Parasite-infected red blood cells sequester in the placenta through interaction between parasite-expressed protein VAR2CSA and the glycosaminoglycan chondroitin sulfate A (CS) abundantly present in the intervillous space. Here, we report cryo-EM structures of the VAR2CSA ectodomain at up to 3.1 Å resolution revealing an overall V-shaped architecture and a complex domain organization. Compared to other PfEMP1s, the ~310 kDa VAR2CSA ectodomain is relatively conserved among parasites. It is composed of a short N-terminal segment and six Duffy Binding-Like (DBL) domains (DBL1-DBL6) unique to VAR2CSA. Several of the DBL domains are linked by complex inter-domain (ID1-3) regions with limited or no homology among PfEMP1s yielding a DBL1-ID1-DBL2-ID2-DBL3-DBL4-ID3-DBL5-ID4-DBL6 structure.

The extracellular region from the N-terminal methionine (M1) to amino acid F2649 representing the entire ectodomain of the FCR3 VAR2CSA variant was expressed in baculovirus transfected insect cells as a secreted monomeric protein and purified by immobilized nickel affinity chromatography. As the binding to CSPG in NaCl buffer showed a 1:2 stoichiometry compared to a 1:1 in KCl buffer, the less compact VAR2CSA could introduce more unspecific binding or the proposed additional minor groove binding site is more exposed in NaCl buffer allowing CSPG binding. Structural analysis was performed in KCl buffer, as the highest affinity toward CSPG was observed. Next, we determined the cryo-EM structure of the isolated VAR2CSA form generated from a map of overall 3.8 Å resolution. The final model represents the ectodomain of VAR2CSA, exhibiting a well-folded conformation with clearly defined DBL domains and in agreement with previously published structures of DBL3, DBL4 and DBL6. The region spanning ID1-DBL2-ID2-DBL3-DBL4-ID3 represents the core of the macromolecular structure, as highlighted by a compact structure with a high degree of inter-domain interactions. The structure discloses the fold of ID2, forming a separate domain consisting of a bundle of α-helices, a shape which together with ID3, a 30 residues long α-helix (residue 1955-1985), serves as a structural glue for the core. Notably, ID2 and ID3 interact, as the C-terminus of ID2 forms an open-mouth shape conformation, which interacts extensively with the ID3 α-helix. DBL1 exhibits only a few inter-domain interaction sites with DBL2 and DBL4, leaving a cleft in-between the core and DBL1. The similarity of the VAR2CSA FCR3 apo-structures by Ma et al., and the one presented here is high, with RMSD in the core region (AA residue 450–2022) of 1.38 Å.

> MDSTSTIANKIEEYLGAKSDDSKIDELLKADPSEVEYYRSGGDGDYLKNNICKITVNHSDSGKYDPCEKKLPPYDDNDQWKCQQNSSDGSGKPENICVPPRRERLCTYNLENLKFDKIRDNNAFLADVLLTARNEGEKIVQNHPDTNSSNVCNALERSFADLADIIRGTDQWKGTNSNLEKNLKQMFAKIRENDKVLQDKYPKDQKYTKLREAWWNANRQKVWEVITCGARSNDLLIKRGWRTSGKSDRKKNFELCRKCGHYEKEVPTKLDYVPQFLRWLTEWIEDFYREKQNLIDDMERHREECTREDHKSKEGTSYCSTCKDKCKKYCECVKKWKTEWENQENKYKDLYEQNKNKTSQKNTSRYDDYVKDFFEKLEANYSSLENYIKGDPYFAEYATKLSFILNPSDANNPSGETANHNDEACNCNESGISSVGQAQTSGPSSNKTCITHSSIKTNKKKECKDVKLGVRENDKDLKICVIEDTSLSGVDNCCCQDLLGILQENCSDNKRGSSSNDSCDNKNQDECQKKLEKVFASLTNGYKCDKCKSGTSRSKKKWIWKKSSGNEEGLQEEYANTIGLPPRTQSLYLGNLPKLENVCEDVKDINFDTKEKFLAGCLIVSFHEGKNLKKRYPQNKNSGNKENLCKALEYSFADYGDLIKGTSIWDNEYTKDLELNLQNNFGKLFGKYIKKNNTAEQDTSYSSLDELRESWWNTNKKYIWTAMKHGAEMNITTCNADGSVTGSGSSCDDIPTIDLIPQYLRFLQEWVENFCEQRQAKVKDVITNCKSCKESGNKCKTECKTKCKDECEKYKKFIEACGTAGGGIGTAGSPWSKRWDQIYKRYSKHIEDAKRNRKAGTKNCGTSSTTNAAASTDENKCVQSDIDSFFKHLIDIGLTTPSSYLSNVLDDNICGADKAPWTTYTTYTTTEKCNKERDKSKSQSSDTLVVVNVPSPLGNTPYRYKYACQCKIPTNEETCDDRKEYMNQWSCGSARTMKRGYKNDNYELCKYNGVDVKPTTVRSNSSKLDGNDVTFFNLFEQWNKEIQYQIEQYMTNANISCIDEKEVLDSVSDEGTPKVRGGYEDGRNNNTDQGTNCKEKCKCYKLWIEKINDQWGKQKDNYNKFRSKQIYDANKGSQNKKVVSLSNFLFFSCWEEYIQKYFNGDWSKIKNIGSDTFEFLIKKCGNNSAHGEEIFSEKLKNAEKKCKENESTDTNINKSETSCDLNATNYIRGCQSKTYDGKIFPGKGGEKQWICKDTIIHGDTNGACIPPRTQNLCVGELWDKSYGGRSNIKNDTKELLKEKIKNAIHKETELLYEYHDTGTAIISKNDKKGQKGKNDPNGLPKGFCHAVQRSFIDYKNMILGTSVNIYEHIGKLQEDIKKIIEKGTPQQKDKIGGVGSSTENVNAWWKGIEREMWDAVRCAITKINKKNNNSIFNGDECGVSPPTGNDEDQSVSWFKEWGEQFCIERLRYEQNIREACTINGKNEKKCINSKSGQGDKIQGACKRKCEKYKKYISEKKQEWDKQKTKYENKYVGKSASDLLKENYPECISANFDFIFNDNIEYKTYYPYGDYSSICSCEQVKYYKYNNAEKKNNKSLCYEKDNDMTWSKKYIKKLENGRSLEGVYVPPRRQQLCLYELFPIIIKNEEGMEKAKEELLETLQIVAEREAYYLWKQYNPTGKGIDDANKKACCAIRGSFYDLEDIIKGNDLVHDEYTKYIDSKLNEIFGSSNTNDIDTKRARTDWWENETITNGTDRKTIRQLVWDAMQSGVRYAVEEKNENFPLCMGVEHIGIAKPQFIRWLEEWTNEFCEKYTKYFEDMKSKCDPPKRADTCGDNSNIECKKACANYTNWLNPKRIEWNGMSNYYNKIYRKSNKESEDGKDYSMIMAPTVIDYLNKRCHGEINGNYICCSCKNIGAYNTTSGTVNKKLQKKETECEEEKGPLDLMNEVLNKMDKKYSAHKMKCTEVYLEHVEEQLNEIDNAIKDYKLYPLDRCFDDQTKMKVCDLIADAIGCKDKTKLDELDEWNDMDLRGTYNKHKGVLIPPRRRQLCFSRIVRGPANLRSLNEFKEEILKGAQSEGKFLGNYYKEHKDKEKALEAMKNSFYDYEDIIKGTDMLTNIEFKDIKIKLDRLLEKETNNTKKAEDWWKTNKKSIWNAMLCGYKKSGNKIIDPSWCTIPTTETPPQFLRWIKEWGTNVCIQKQEHKEYVKSKCSNVTNLGAQASESNNCTSEIKKYQEWSRKRSIQWETISKRYKKYKRMDILKDVKEPDANTYLREHCSKCPCGFNDMEEMNNNEDNEKEAFKQIKEQVKIPAELEDVIYRIKHHEYDKGNDYICNKYKNIHDRMKKNNGNFVTDNFVKKSWEISNGVLIPPRRKNLFLYIDPSKICEYKKDPKLFKDFIYWSAFTEVERLKKAYGGARAKVVHAMKYSFTDIGSIIKGDDMMEKNSSDKIGKILGDTDGQNEKRKKWWDMNKYHIWESMLCGYREAEGDTETNENCRFPDIESVPQFLRWFQEWSENFCDRRQKLYDKLNSECISAECTNGSVDNSKCTHACVNYKNYILTKKTEYEIQTNKYDNEFKNKNSNDKDAPDYLKEKCNDNKCECLNKHIDDKNKTWKNPYETLEDTFKSKCDCPKPLPSPIKPDDLPPQADEPF> MRAEARGGLERFCSAGKGRGLRALRPFHVGDLLFSCPAYACVLTVGERGHHCECCFARKEGLSKCGRCKQAFYCDVECQKEDWPLHKLECSSMVVLGENWNPSETVRLTARILAKQKIHPERTPSEKLLAVREFESHLDKLDNEKKDLIQSDIAALHQFYSKYLEFPDHSSLVVLFAQVNCNGFTIEDEELSHLGSAIFPDVALMNHSCCPNVIVTYKGTLAEVRAVQEIHPGDEVFTSYIDLLYPTEDRND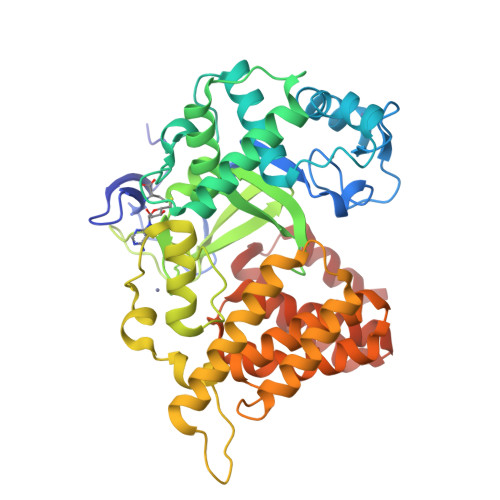RLRDSYFFTCECRECTTKDKDKAKVEVRKLSSPPQAEAIRDMVRYARNVIEEFRRAKHYKSPSELLEICELSQEKMSSVFEDSNVYMLHMMYQAMGVCLYMQDWEGALKYGQKIIKPYSKHYPVYSLNVASMWLKLGRLYMGLENKAAGEKALKKAIAIMEVAHGKDHPYISEIKQEIESH4-[(5-bromanyl-4,6-dimethyl-pyridin-2-yl)amino]-4-oxidanylidene-butanoic acid | C11 H13 Br N2 O3 | 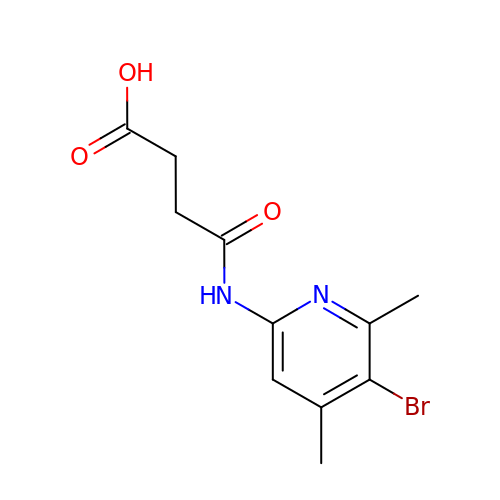AYWBCWUDJKSIMU-UHFFFAOYSA-N> GPAMAKVETGTDVTSKVTVEIGSIEGHNNTNKVEPHAGQRAVLKYKLKFENGLHQGDYFDFTLSNNVNTHGVSTARKVPEIKNGSVVMATGEVLEGGKIRYTFTNDIEDKVDVTAELEINLFIDPKTVQTNGNQTITSTLNEEQTSKELDVKYKDGIGNYYANLNGSIETFNKANNRFSHVAFIKPNNGKTTSVTVTGTLMKGSNQNGNQPKVRIFEYLGNNEDIAKSVYANTTDTSKFKEVTSNMSGNLNLQNNGSYSLN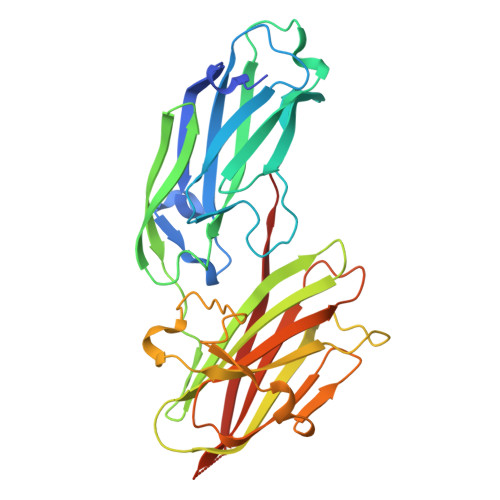IENLDKTYVVHYDGEYLNGTDEVDFRTQMVGHPEQLYKYYYDRGYTLTWDNGLVLYSNKA>GSHMDPF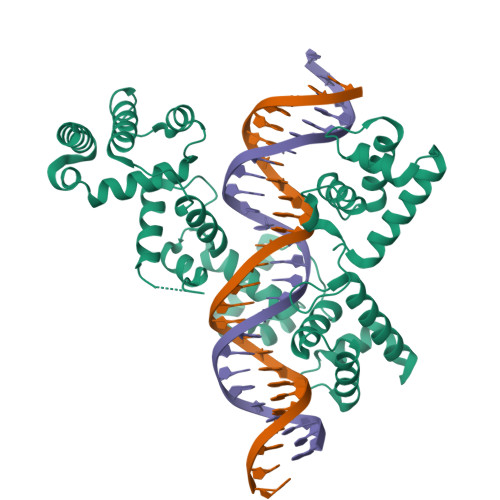LKGSARWTAEHWDYLERRMQNFCQTYSLDHTQVADSLHEKRLHGPLSSLVKLLVQEMPSFTRRTILRHLRALYNIPGYEKYSRKNSSGRGDFGVQETAIISQEVHNFIMDQGWSEYQFCNQIWAGKCPKTIRMFYSNLYKKLSHRDAKSIYHHVRRAYNPFEDRCVWSKEEDEELRKNVVEHGKCWTKIGRKMARMPNDCRDRWRDVVRFGDKLKRNAWSLEEETQLLQIVAELRNREDLSSDINWTLVAQMLGTRTRLQCRYKFQQLTKAASKFELQENVWLLERIYDSLLNNGGKIHWENIVKEANGRWTRDQMLFQFINLKKMIPSYDNLPLLEATKSAIDDFKVVLSGFSN[2x]> DVVVQAPTQVPGFLGDSVTLPCYLQVPNMEVTHVSQLTWARHGESGSMAVFHQTQGPSYSESKRLEFVAARLGAELRNASLRMFGLRVE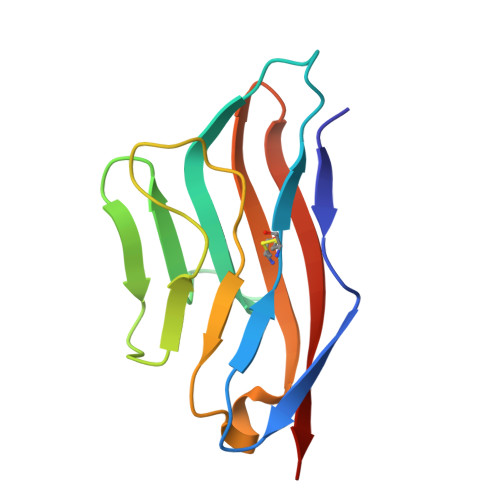DEGNYTCLFVTFPQGSRSVDIWLRVLAKP>[6x]MRGS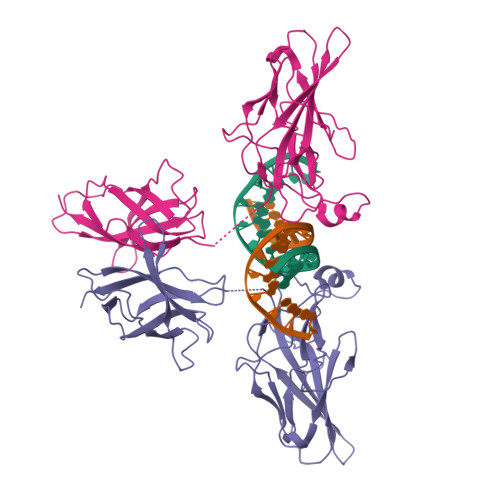HHHHHHTDPHASSVPLEWPLSSQSGSYELRIEVQPKPHHRAHYETEGSRGAVKAPTGGHPVVQLHGYMENKPLGLQIFIGTADERILKPHAFYQVHRITGKTVTTTSYEKIVGNTKVLEIPLEPKNNMRATIDCAGILKLRNADIELRKGETDIGRKNTRVRLVFRVHIPESSGRIVSLQTASNPIECSQRSAHELPMVERQDTDSCLVYGGQQMILTGQNFTSESKVVFTEKTTDGQQIWEMEATVDKDKSQPNMLFVEIPEYRNKHIRTPVKVNFYVINGKRKRSQPQHFTYHPV>[5x]GAMATEQIQHIAIVGCVH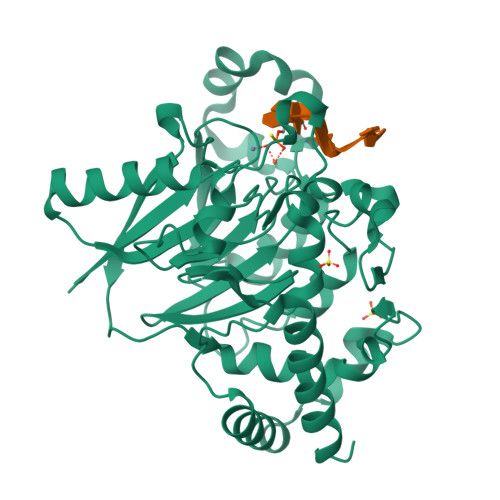GKYREMYRQLSEYEKSTGKEISFVICTGDMQTLRYEADLVYLKVPPKYKQMGDFHLYYEGKEKAPYLTLFIGGNHESSNVLLHLYNGGFVCFNMYYLGVCSCININGLRIVGVSGIYKSFDEKKPYTYPPSPNDVVSLFHTRNYVIQMLSNLSQSSQIDISLSHDWPQGIVMKGNYKQLYRFQPGFKKDGASLGSPINKVILNTLKPKYWISGHMHCEYHAEEGPTHFIALGKIGYKNAISYLDLPLKQKTDLEYDKDWVCNLIMTWPAFSNKAQFPDLSYSISELLSKRTKELDKKIIELWEKYIGLKIIYDSDTFDIQFTSRRFYIEKIYNELNIN> ASMEINVSKLRTDLPQVGVQPYRQVHA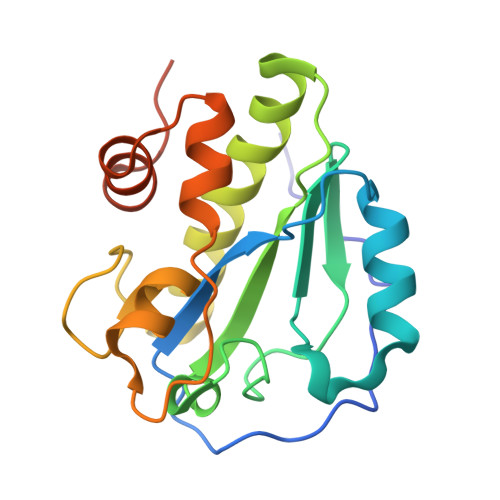HSTGNPHSTVQNEADYHWRKDPELGFFSHIVGNGAIMQVGPVDNGAWDVGGGWNAETYAAVELIESHSTKEEFMTDYRLYIELLRNLADEAGLPKTLDTGSLAGIKTAEYATNNQPNNHSDHVDPYPYLAKWGISREQFKHDIENGLTIETGWQKHHHHHH> MSLSALESSSRFEVRYFFERALECYKPFSDTVLLLPCTARKPYLTSRTHRALRSKVKVN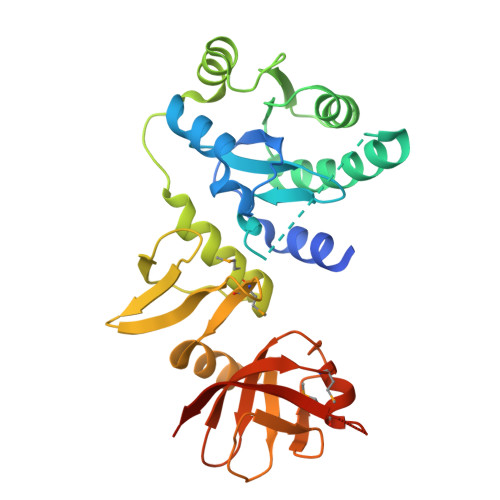VNEIIISSPLVVPREFELLYPAVNYDTPVTGHWSEEEVSFVAGWLKRFIEKGGFRKVVAHVTGGYRKVVERVEDEVEAEVVYTAEKDVLSDESIERLKQEIESKGKVDLYRRILEHMLSYQFGITWSGKVAGRYPELELLEGKKRLARVDRIYGMLDIYEKIAAYLLEKNIYTVEIGDFEVKGTIFAGGVLRADEKIRPNDVVVFHNSRIFGVGLAAMSGKEMAGSEKGIAINVKRKFSEGHHHHHH> IVGGTESSWGEWPWQVSLQVKLTAQRHLCGGSLIGHQWVLTAAHCFDGLPLQDVWRIYSGILELSDITKDTPFSQIKEIIIHQNYKVSEGNHDIALIKLQAPLEYTEFQKPISLPSKGDTSTIYTNCWVTGWGFSKEKGEIQNILQKVNIPLVTNEECQKRYQDYKITQRMVCAGYKEGGKDACKGDSGGPLVCKHNGMWRLVGITSWG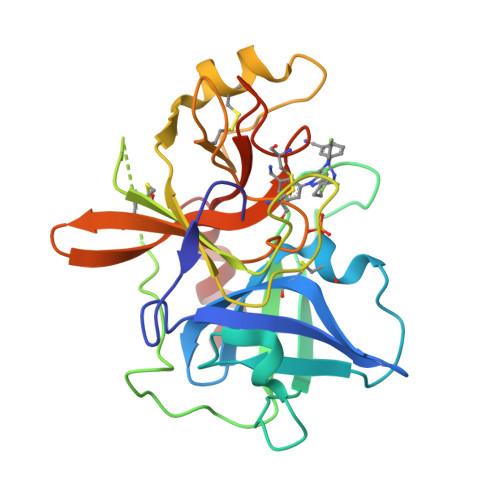EGCARREQPGVYTKVAEYMDWILEKTQ> DCGLPPDVPNAQPALEGRTSFPEDTVITYKCEESFVKIPGEKDSVICLKGSQWSDIEEFCNRSCEVPTRLNSASLKQPYITQNYFPVGTVVEYECRPGYRREPSLSPKLTCLQNLKWSTAVEF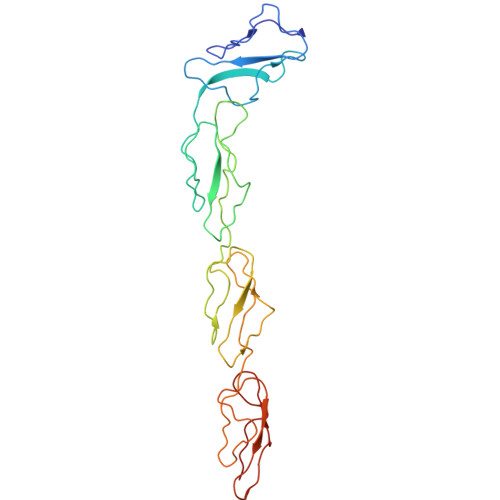CKKKSCPNPGEIRNGQIDVPGGILFGATISFSCNTGYKLFGSTSSFCLISGSSVQWSDPLPECREIYCPAPPQIDNGIIQGERDHYGYRQSVTYACNKGFTMIGEHSIYCTVNNDEGEWS>MAFEENLYCDYTPGAAKAVAGKDVILAVFNAAGDKLLAVAGQQGLTVNRSKDSIEITSKDTVGGWKSKIGGMKEWSIENDGLYVADAESHKELAKYFESDSPVCVKIINQASKKGLFGGLAIVADYSFEAPFDEAMTYSVKL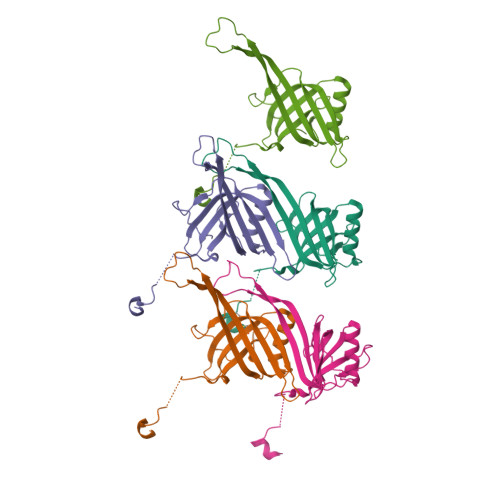DGMGALVDLTITEGGDQMPGETPVAPAE[5x]>[2x]GHMADKIKNAKIVFVVGGPGSGKGTQCEKIVAKYGYTHLSSGDLLRAEVASGSERGKQLQAIMQKGELVPLDTVLDMIKDAMIAKADVSKGYLIDGYPREVKQGEEFEKKIGAPALLLYIDAKGETMVKRLMKRGETSGRADDNEETIKKRLDLYYKATEPVIAFYEQRGIVRKINSELPVDEVFAIVEKAIDELK

AK is a small enzyme that catalyzes a reversible phosphoryl transfer reaction between ATP/AMP and two ADPs. The structures comprised the characteristic three-domain arrangement: the CORE (residues 1–38, 69–136, and 143–193), AMPbind (residues 39–68), and LID (residues 137–142) domains. The static CORE domain provides substrate-binding sites, and the dynamic AMPbind and LID domains close over the AMP and ATP sites, respectively, upon substrate binding. AK is a small protein that undergoes relatively large conformational changes upon substrate binding and product release, and has long been used as a model system for studying connections between structure, function, and dynamics.

To assess the structural basis of cold adaptation, we determined the crystal structures of AKNc and AKDr to resolutions of 1.99 and 1.75 Å, respectively, using molecular replacement. Among the tropical AKs, AKDr was the most thermally stable. The three AKs from the tropical fishes including AKDr have Ile28, Ala48, and Lys188 at these positions, whereas AKNc has Val28, Ser48, and Thr188. In the structure of AKDr, the longer side chain of Ile28 enhances the hydrophobic contacts with the residues in β3 and α9, and interacts more closely with hydrophobic residues in β1 and β4. At these positions, AKXm and AKPr also have Val residues, but AKDr, which is the most thermally stable of the three tropical AKs, has Ile residues. In the crystal structure of AKDr, Ile118 and Ile173 improve CORE packing cooperatively by increasing hydrophobic interactions between them as well as with other residues. We produced an AKDr mutant in which Ile28, Ile118 and Ile173 residues were replaced with Val residues, and determined its Tm value. The reverse triple mutation significantly reduced the thermal stability of AKDr, as indicated by a decrease in Tm of 8.9 °C relative to the WT enzyme, confirming the importance of the CORE packing in the overall stability of the fish AKs. The AKDr mutant exhibited increased catalytic activities at low temperatures (5 °C and 35 °C) compared to the WT enzyme, and the temperature of maximum activity decreased (35 °C). In the crystal structure of AKDr, we identified a salt bridge connecting between Arg171 and Glu192, which is substituted to Ala192 in AKNc.>MASDKFPVAENPSSSFKYESAVQYRPAPDSYLNPCPQAGRIVKETYTGINGTKSLNVYLPYGYDPNKKYNIFYLMHGGGENENTIFSNDVKLQNILDHAIMNGELEPLIVVTPTFNGGNCTAQNFYQEFRQNVIPFVESKYSTYAESTTPQGIAASRMHRGFGGFAMGGLTTWYVMVNCLDYVAYFMPLSGDYWYGNSPQDKANSIAEAINRSGLSKREYFVFAATGSEDIAYANMNPQIEAMKALPHFDYTSDFSKGNFYFLVAPGA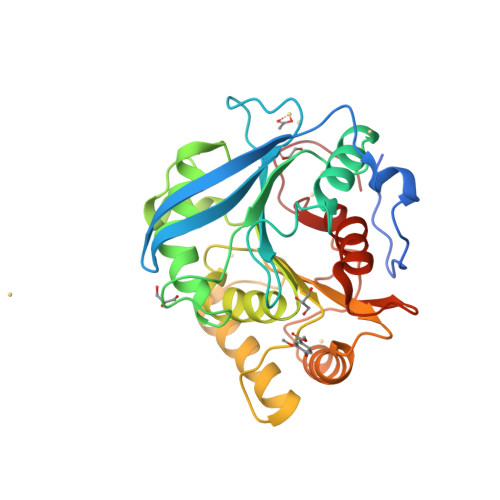THWWGYVRHYIYDALPYFFHELEHHHHHH[2x]>MRRYNTGLFLLSMVMLAGCGKPEVNVVMTGDMTTRLAFAGEQLKQALVEKGYEVNQTTDEKEIGGGKRSIYLNLLNDTTKKNKERFDISTKGKNTYVTGYDGNGIIYGCRELIDQLDQSGTMDFKPVSDAPEMVLRGACIGLQKTTYLPGHAVYEYPYTPESFPWFYDKERWIKYLDMMVENRMNSLYLWNGHPFASLVKLKDYPFALEVDEETFKKNEEMFSFLTTEAEKRGIFVIQMFYNIIVSKPFADHYGIKTQDRNRPITPLISDYTRKSVAAFIEKYPNVGLLVCLGEAIGTYEEDVEWFTKTIIPGIKDGLKVLGRTDEPPVLVRAHDTDCKMVIDAALPLYKNLYTMHKYNGSSLTTYEPRGPWAKIHKDLSSLGSVHISNVHILANLEPWRWSSPDFIQKSVKAMHSVHGANALHIYPQANYWDWPYTADKLANGEREEQVYRDWAWYKAWGRYAWKADRNRLEEIKYWDKQFGDFYGIPAEMADNIRIAYEESGEIAPKLLRRFGITEGNRQ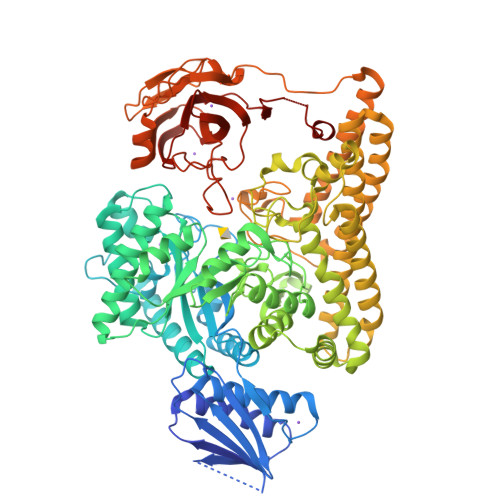TLLLGMFMSQFVNPYKYTIHYGFYESCGPGGEKLIEYVEKEWKKQPHVGELPLDIINQVIEHGDKAVAAIDKVVSSAKKNSDELRRLQNDMHCYREYAYAFYYKVKAAQHVLNYHWGKNMDELDKAVPLMEESLKHYTKLVDLTKDTYLFANSMQTAQRRIPIGGDDGNNKTWSEMLVHYKAELYNFKENIEMLKDKKVRKCVEVTPLKEADVKILNNLTKVKIEKGAKIFSNIDGGIDAIAKEITGLTGFVFNGEKQRDDATTIEFECSSPVTMLVAYFKDDHRKFAKAPRLESDASANDYGQAEPVLTNALHVKGVALADIYPYKFKAGRHTLILPKGYCGVLGFTEDKIKERDVALEGGADAPDWLFY[2x]> RNIIXG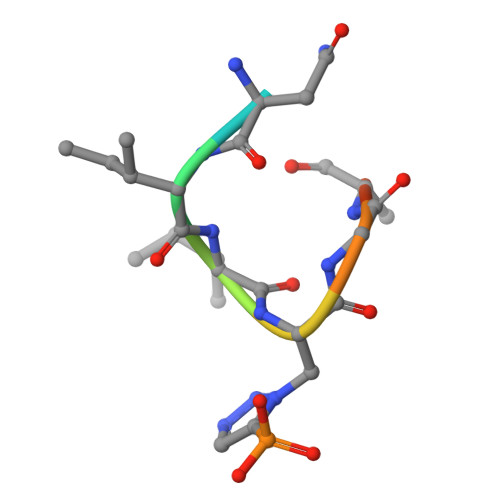SDS(E,4S)-4-[[5-[2-[2,6-bis(azanyl)-4-oxidanylidene-1H-pyrimidin-5-yl]ethanoylamino]-3-fluoranyl-pyridin-2-yl]carbonylamino]pent-2-enedioic acid | C17 H18 F N7 O7 | 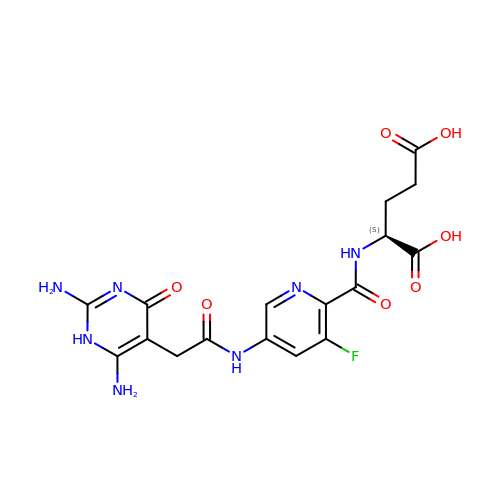ALGPVOJFIGPPPX-VIFPVBQESA-N>[2x]XGEIAQAIKE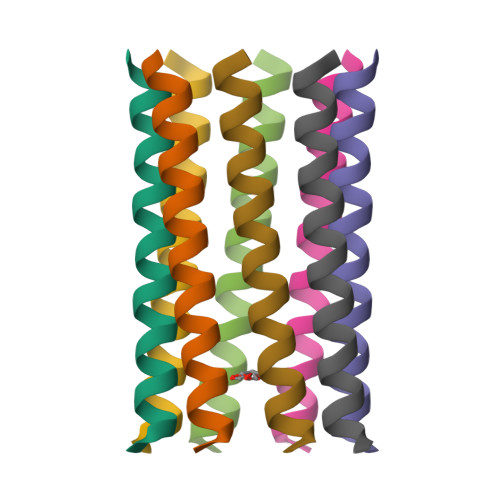IAKAIKEIAWAIKEIAQAIKGX> GPLGSMSEEQVAQDTEEVFRSYVFYRHQQEQEAEGVAAPADPEMVTLPLQPSSTMGQVGRQLAIIGDDINRRYDSEFQTMLQHLQPTAENAYEYFTKIATSLFESGINWGRVVALLGFGYRLALHVYQHGLTGFLGQVTRFVVDFMLHHSIARWIAQRGG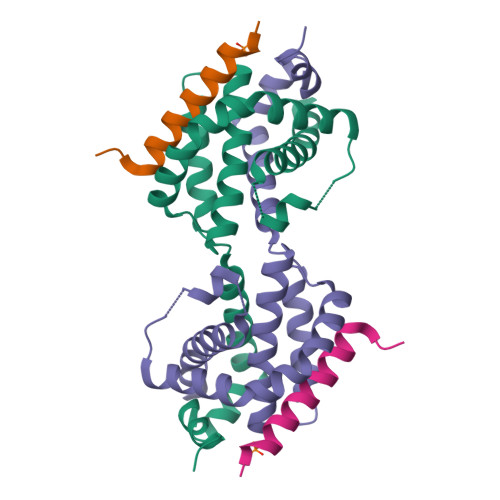WVAALNLGNG;> DMRPEIRIAQELRRXGDEFNATYARR> DRKRRSDPNFKNRLRERRKKQKLAKERAGLSKLPDLKDAEAVQKFFLEEIQLGEELLAQGEYEKGVDHLTNA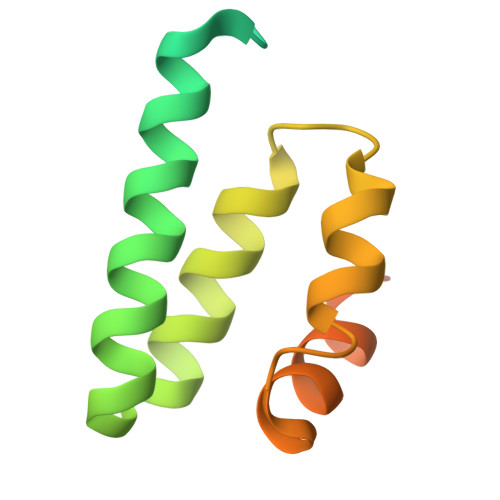IAVCGQPQQLLQVLQQTLPPPVFQMLLTKLPTISQRIVSAQSLAEDDVE> GPGSTVKDNSLLFMPNVLKVYLENGQTKSFRFDCSTSIKDVILTLQEKLSIKGIEHFSLMLEQRTEGAGTKLLLLHEQETLTQVTQRPSSHKMRCLFRISFVPKDPIDLLRRDPVAFEYLYVQSCNDVVQERFGPELKYDIALRLAALQMYI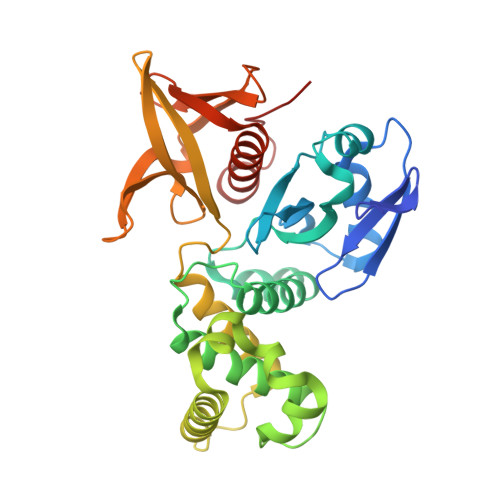ATVTTKQTQKISLKYIEKEWGLETFLPSAVLQSMKEKNIKKALSHLVKANQNLVPPGKKLSALQAKVHYLKFLSDLRLYGGRVFKATLVQAEKRSEVTLLVGPRYGISHVINTKTNLVALLADFSHVNRIEMFSEEESLVRVELHVLDVKPITLLMESSDAMNLACLTAGYYRLLVDSRRSIFNMAN> MQAFGVLDRYIGKTIFTTIMMTLFMLVSLSGIIKFVDQLKKAGQGSYDALGAGMYTLLSVPKDVQIFFPMAALLGALLGLGMLAQRSELVVMQASGFTRLQVALSVMKTAIPLVLLTMAIGEWVAPQGEQMARNYRAQAMYGGSLLSTQQGLWAKDGQNFVYIERVKGDDELGGVSIYAFNDERRLQSVRHASSAKFDPEHKQWRLSQVDESDLTNPKQITGSQTVSGTWKTNLTPDKLGVVALDPDALSISGLHNYVKYLKSSGQDAGRYQLN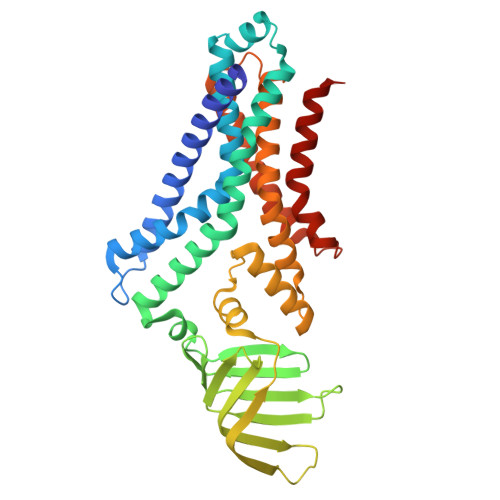MWSKIFQPMSVAVMMLMALSFIFGPLRSVPMGVRVVTGISFGFVFYVLDQIFGPLTLVYGIPPIIGALLPSASFLLISLWLLLKRS N-({1-[(1R,2R,4S)-bicyclo[2.2.1]hept-2-yl]-1,6-dihydroimidazo[4,5-d]pyrrolo[2,3-b]pyridin-2-yl}methyl)methanesulfonamide 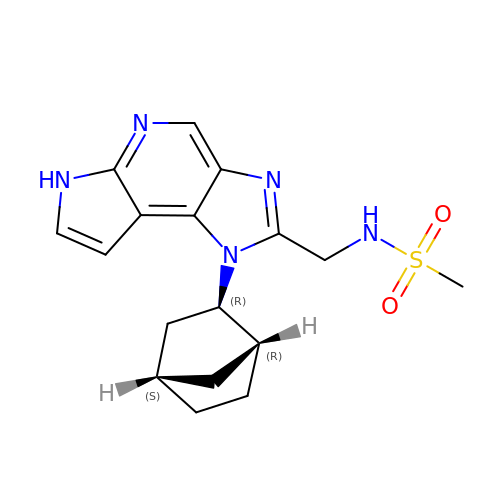| C17 H21 N5 O2 S | IQHKHGHDPGFXAV-MISXGVKJSA-N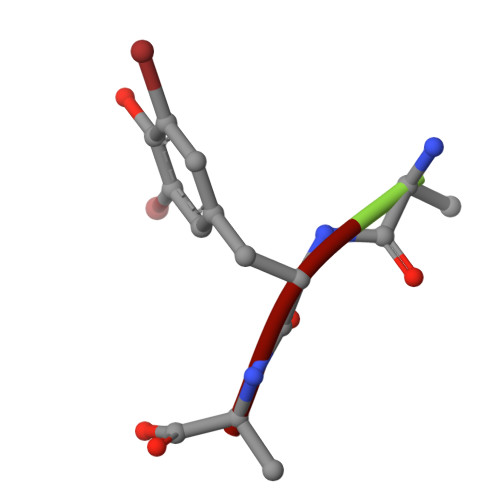> AYA> GESELSSNPAASAGASLEPPAAPAPGEDNPAGAGGAAVAGAAGGARRFLCGVVEGFYGRPWVMEQRKELFRRLQKWELNTYLYAPKDDYKHRMFWREMYSVEEAEQLMTLISAAREYEIEFIYAISPGLDITFSNPKEVSTLKRKLDQVSQFGCRSFALLFDDIDHNMCAADKEVFSSFAHAQVSITNEIYQYLGEPETFLFCPTEYCGTFCYPNVSQSPYLRTVGEKLLPGIEVLWTGPKVVSKEIPVESIEEVSKIIKRAPVIWDNIHANDYDQKRLFL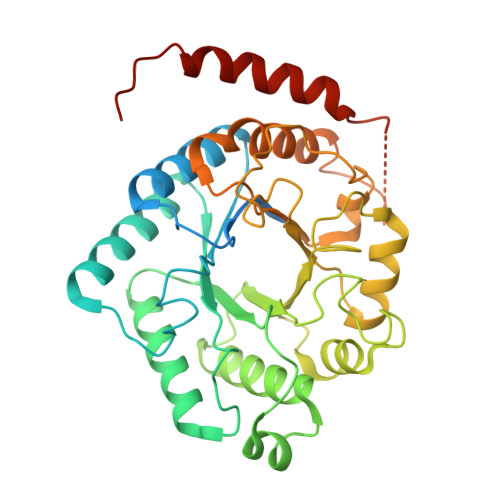GPYKGRSTELIPRLKGVLTNPNCEFEANYVAIHTLATWYKSNMNGVRKDVVMTDSEDSTVSIQIKLENEGSDEDIETDVLYSPQMALKLALTEWLQEFGVPHQYSSR> GAACGACAGTGA;> CGTCGACTC;> TCAACG;> TCGAGTCGCTGTCGT

In this work, we exhaustively probe the ability of all 36 immobile HJ sequences to form DNA crystals in two different designed systems. Three separate self-assembling DNA crystal systems are described in this report: the “4 × 5” and “4 × 6” designs (collectively referred to as the 4 × N systems), and a third construct with a “scrambled” sequence variant of the 4 × 6 lattices. Self-assembly was mediated by three constituent oligonucleotides: (S1) containing four sequence repeats of either 5 or 6 bases; (S2) composed of 21 bases containing complementary regions to both (S1); and (S3) which forms the second junction crossover. The HJ serves as the fundamental component at the core of each unit, and the ultimate assembly of the full lattice is facilitated by the complementary 2-base sticky ends that tail each duplex.

To investigate this possibility, we designed “scrambled” sequences with targeted base substitutions, while maintaining GC content, along each “stem”. Contrary to the buffer preference observed with the native P32 crystals, the scrambled systems exhibited an exclusive preference towards low salt buffers, much like the native R3 crystals. Remarkably, only J1 and J2 retained the P32 symmetry, with all others yielding an R3 lattice. There appeared to be only a marginal difference in the average cell lengths in the R3 scramble crystals (a = b = 113.04 c = 51.10) relative to the native 4 × 6 sequences: the a, b axis trended ~2 Å shorter and c ~1.3 Å longer, whereas in the J1 and J2 cases, the crystals were in good agreement with the original 4 × 6 motif. The average angles of the R3 and P32 crystals were 61.00° (σ = 1.21) and 58.05° (σ = 1.39), respectively. Further, we observed modest improvements in resolution, reaching as high as 2.7 Å in J36. Notably, all junctions preventing crystallization compared to its original counterpart remained fatal and all relative cavity dimensions and volumes remained unperturbed. However, in the majority of the crystal structures reported here, the cacodylate anion indeed fits best into the electron density map of our X-ray structures, due to the presence of sodium cacodylate in the crystallization solution.>[3x]M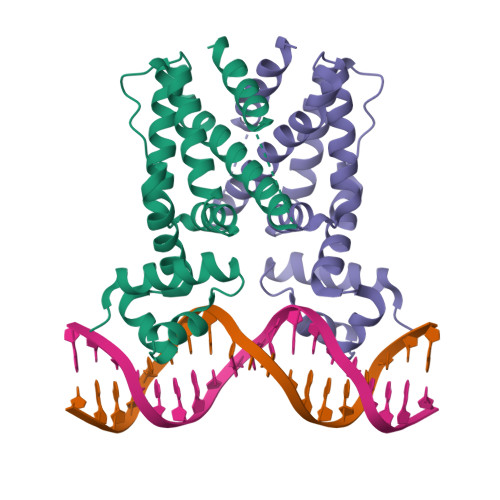GSHHHHHHSSGLVPRGSHSDEVDAHMVQLHKPDVVAAATKILDDHGIADLTMRRLARELDVTPGALYWHFANKQELLGAVADHILRTARTDTADLAWREQIHESCRALRDALLSHTDGAELVSASFASGQSVVITEIVEQLGRAARAAGVSDADVDAAARTVIYYVLGFTVDEQSRLQWDAVGALGDDQSMLTRDGTRQFRFGLQLLVDGLAAHGGGSEFTGFSSAERSFE> GPDHMSRLEIYSPEGLRLDGRRWNELRRFESSINTHPHAADGSSYMEQGNNKIITLVKGPKEPRLKSQMDTSKALLNVSVNITKFSKFERSKSSHKNERRVLEIQTSLVRMFEKNVMLNIYPRTVIDIEIHVLEQDGGIMGSLINGITLALIDAGISMFDYISGISVGLYDTTPLLDTNSLEENAMSTVTLGVVGKSEKLSLLLVEDKIPLDRLENVLAIGIAGAHRVRDLMDEEL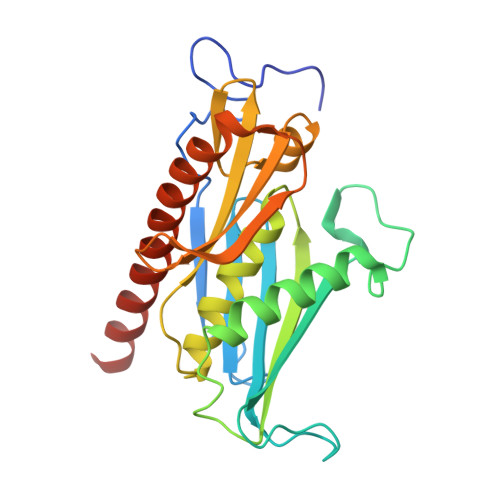RKHAQKRVSNASAR> RRKKPQDHFFDVPAEED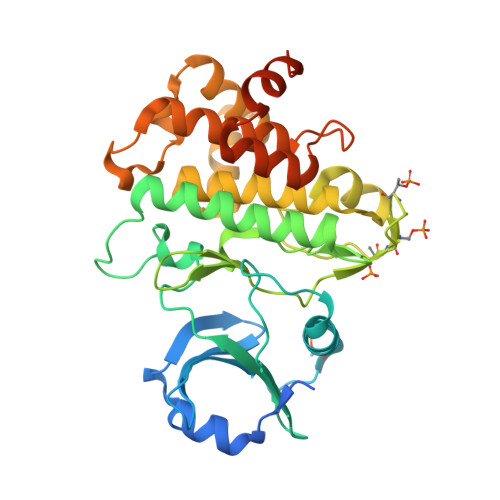PEVHLGQLKRFSLRELQVASDNFSNKNILGRGGFGKVYKGRLADGTLVAVKRLKEERTQGGELQFQTEVEMISMAVHRNLLRLRGFCMTPTERLLVYPYMANGSVASCLRERPESQPPLDWPKRQRIALGSARGLAYLHDHCDPKIIHRDVKAANILLDEEFEAVVGDFGLAKLMDYKDTHVTTAVRGTIGHIAPEYLSTGKSSEKTDVFGYGVMLLELITGQRAFDLARLANDDDVMLLDWVKGLLKEKKLEALVDVDLQGNYKDEEVEQLIQVALLCTQSSPMERPKMSEVVRMLEGDGLAERWEEWQKEEMFRQDFNYPTHLEHHHHHH>GPGSMAATPLPPLRLAIACDDAGVSYKEALKAHLSDNPLVSSITDVGVTSTTDKTAYPHVAIQAAQLIKDGKVDRALMICGTGLGVAISANKVPGIRAVTAHDTFSVERAILSNDAQVLCFGQRVIGIELAKRLAGEWLTYRFDQKSASAQKVQAISDYEKKFVEVN[2x]

Ribose-5-phosphate isomerases catalyze the interconversion of ribulose-5-phosphate and ribose-5-phosphate as an important part of the pentose phosphate pathway. Two types of ribose-5-phosphate isomerases exist, RpiA and RpiB, which share little structural homology and have distinct active sites and mechanisms of action. Although RpiB occurs predominantly in bacteria, here we report crystal structures of a putative RpiB from the pathogenic fungus Coccidioides immitis. The C. immitis RpiB contains the canonical open (α,β) Rossman fold, a common fold for proteins that bind nucleotides or nucleotide-like molecules.

A 1.9 Å resolution apo structure was solved by combined molecular replacement and single wavelength anomalous dispersion (SAD) phasing using a crystal soaked briefly in a solution containing a high concentration of iodide ions. Given that the C. immitis RpiB contains modest sequence identity to other structurally characterized RpiBs, we attempted to solve the crystal structure of C. immitis RpiB by iodide ion single wavelength anomalous dispersion (SAD) phasing, a strategy that has proven successful for structure determination of many SSGCID targets. Attempts to solve the structure by molecular replacement with other RpiBs such as that from Clostridium thermocellum yielded clear rotation and translation solutions, yet poor refinement statistics (R of 0.39 and Rfree 0.47). Therefore the partial molecular replacement solution was combined with the SAD phases and yielded a clearly interpretable electron density map (FOM 0.53 prior to density modification) into which Buccaneer built both molecules in the asymmetric unit end-to-end in less than one minute. Interestingly, the active site contains electron density consistent with an oxidized cysteine residue (Cys76) in both protomers. Although the exact oxidation state of the cysteine residue was not determined, the electron density maps were most consistent with two conformations of the sulfenic state rather than sulfinic or sulfonic acid. The oxygen on Cys76 appears to adopt two different orientations contacting the backbone nitrogen and side chain hydroxyl of Thr78 in one orientation and the backbone nitrogens of Gly81 and Val82 in the other. The oxidized nature of Cys76 may imply that this residue, thought to be the catalytic base, is highly reactive. The high concentration solution of sodium iodide used for phasing likely contains iodine, indicated by a light yellow color. Iodine is the most probable source for the oxidation of Cys76, which was not oxidized in the other two C. immitis RpiB structures (see below). An iodide ion resides in the same place as this chloride ion in both protomers of the asymmetric unit in the iodide-phased structure.> MSIIKDVQDSNDPQLDKFNNEDAPKLAPVIPTPQPTDAGLSLGSTPVGVNPQAVIETESTPQPLTPEQQALTDSYNEASRLTTNVQPMSELVQPQQALPTPTNIDSQQPTVFESANQFNLSATDNLLQQGKITQELINETQLTQSHIPTVYST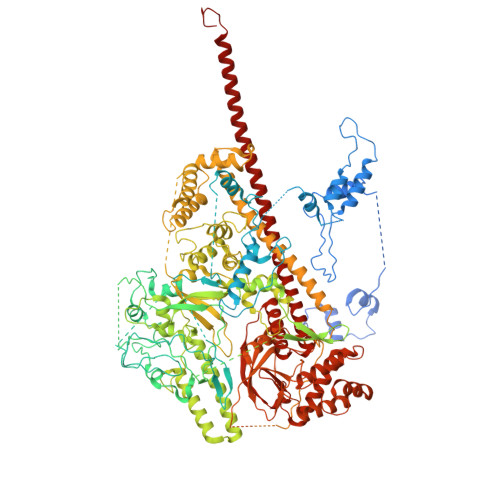PYDGDEWDLDFEASLERAGVLPGQKPSPETFNSQFNAQPTNEDASRSFNPNALKRSQFDVEGALAAIRNINTQEGLTGYQTIKPWGEGALSSLMYGLGVVSNTIRGGVIDAVNVRNRVVNQLPKPIQGVLNFNPASALTGQQLIRPDANYRGSYTLDAIRGRQYSFTANSTNKDEPIGITGFKAFDDLAERMRQNRNARYNAINKTFGREIAKPVAVEERWSTDLSFWAGFGLDTILDPIDSIGVAWKASGLLLGNAPSYVKRGIPTNTGRVIVTPAASERKLLPPGRTRYTPPGKPDGYELGLTEPLTNNKYQVVQTPKGEVSIPVGQPTVQAKLPSIASNNKVTSLTLRREIRRPDGVIDVEFTPNPGAFDRVTGISNEPLAQLPSSEARRPLEPTQFETIQTPNGEVQVPINQPSAPRQLPGTRTYSQPNWRWSRVVDGYINPEGMQPIIEVVRRKPEVFTTNSTSGYSPNWEYWSAPKVDDLYIPAPIDVEFKVIPNKPSNLPLKPSSLSEDIVQGVDGEVRVPSSTQPNSQLALPYGEPYPLTQWDLSLETNPPQIGQRIDNNITVAKNQGEAIDDVINNAPRTVEYNVSGLEIPRRNVTPQGFPKLEPRYDIKPPETPRVIELAPESVTVIREALDSNDWVKAYDELLRKRVPVSDIKRKLETGRIDEAVNDLRKLIGDIKPKTAPEPKPVAPKRQRRRVIKADGTAVYETVRVNPETQLLDAAITNINVVANVVDVPSMSVSQSTPASPLAIDAASDALRPVSPGTPLVAPTSEVNKQLVDQLTRLTETERMMKRRGASPETLERIRTQKLELRKAIADGDELAEPKVKPEPVTPAINKTVLTGTMTMSELSQQLLDNVPGSRIDPDKVRRVERKLSEVEALMKVIPNPITGEPLLGSANTRKFRTWAKDSSTSPTAYLNKLGLQEYPLLYRLFERDGAAIDIDALAHPEFRVILDKPLPDKTSRQVVVSNTPSLTKPTVQSESKAITEMTINELRSERKLLKSQINELDDPSDLIERLMELDDAINNLDITKPENLKVVQDEVIPETQHGTSPEVVKLTQQKLDIENEVINTGVRVQELELELARQKVQLEDALSRIEETADINPHDVISEPLPSGRARRVPTEIPPNDGTILTQKEAARFYDISEGNFKNGDTKPRPALVHTKHMVSDVVVPNDVIQREFDNIMNMGGITQPIVITPVGLDDVYIKYAVVDNHAIYEAAKLAREADPRKFENVNVIVIHPSKADPSYFADEVLPTNTTEGSLYHGTRVKGWTPGNGGVGEWGSGTYFSKSSQAASDNAIKPLRPALGEVIDNVTQPTIHEVLPDFKRTVDVNSPVDGDFSAALLMSANELMDGSEFTSFKRSIMKPGTVQLRDTIKTPADIYAAIEKYAAKNDIEWTPERTHKFKSRINERLRLVGVDALTDGDTTLVINPDAVSVINSHLLDETDAIGTSIARYNSASEAAGRNSGIPTANANQAEASVMLQRQMYEETIEKLEDAKRQQRTAITKSHEIDEQLTQTAQAEQTTKRQQRVAKSQKRAEREAERLGKKRDNPCQF>[2x]SNAMKENNTILKRQDYKIKFNNKDMDFCFNWMLGIGQIIGMSAGELFYIASGIRDGNPTDWCKRFNEHADYLEDEVERVKKVGYRDLISHLYFSACFSIRAALQFTDPKDSEFMENFRRMEKLFMLAVDNSKIPLKSIEVPFEGELLPGYAIISEDKAQDTLIVVGGGDTSREDLFYMLGYSGWEHDYNVLMVDLPGQGKNPNQG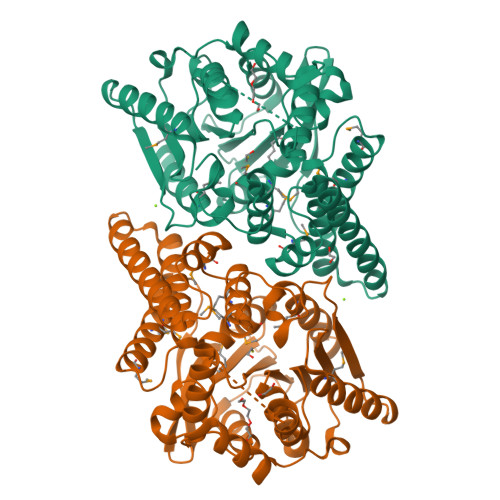LHFEVDARAAISAILDWYQAPTEKIAIAGFSGGGYFTAQAVEKDKRIKAWIASTPIYDVAEVFRISFSTALKAPKTILKWGSKLVTSVNKVAEVNLNKYAWQFGQVDFITSVNEVLEQAQIVDYNKIDVPSLFLVGAGEDSELMRQSQVLYDNFKQRGIDVTLRKFSSESGADAHCQVNNFRLMHYQVFEWLNHIFKKKD> LSDSRVLWAPAEAHPLSPQGHPARLHRIVPRLRDVFGWGNLTCPICKGLFTAINLGLKKEPNVARVGSVAIKLCNLLKIAPPAVCQSIVHLFEDDMVEVWRRSVLSPSEACGLLLGSTCGHWDIFSSWNISLPTVPKPPPKPPSPPAPGAPVSRILFLTDLHWDHDYLEGTDPDCADPLCCRRGSGLPPASRPGAGYWGEYSKCDLPLRTLESLLSGLGPAGPFDMVYWTGDIPAHDVWHQTRQDQLRALTTVTALVRKFLGPVPVYPAVGNHESTPVNSFPPPFIEGNHSSRWLYEAMAKAWEPWLPAEALRTLRIGGFYALSPYPGLRLIS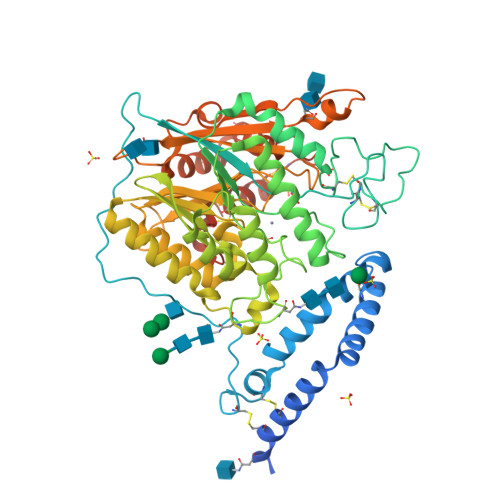LNMNFCSRENFWLLINSTDPAGQLQWLVGELQAAEDRGDKVHIIGHIPPGHCLKSWSWNYYRIVARYENTLAAQFFGHTHVDEFEVFYDEETLSRPLAVAFLAPSATTYIGLNPGYRVYQIDGNYSGSSHVVLDHETYILNLTQANIPGAIPHWQLLYRARETYGLPNTLPTAWHNLVYRMRGDMQLFQTFWFLYHKGHPPSEPCGTPCRLATLCAQLSARADSPALCRHLMPDGSLPEAQSLWPRPLFC> MAHHHHHHMQTYINPPLSEWKNLIQRPVQKAEDLQNIVLTVFEDIKNEKDKALINYTKKFDKAYLTDIRVSSDEITAAIALVSDELIQAIQMAASNIEKFHASQKENKNIIETTEGVNCWREARPIENIGIYIPGGSAPLFSTVLMLGIPAQLAGCKNITLCTPPDESGNINPAILYTANLIGIKNIYKAGGIQAIGAMTFGTETIEKADKIFGPGNQYVTAAKQIAQNFGVAIDMPAGPSEVLVIADTTANPEFVAADLLSQAEHGADSQVILLTTDENILQQTLMQVENQLTQLPRKSIASQALLQSRGIVLDS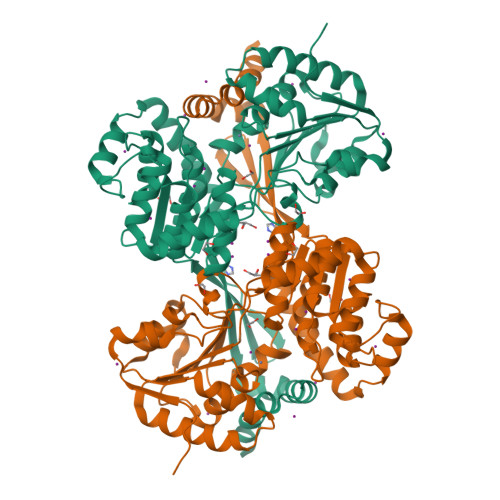IEKCIAFSNLYAPEHLILAIENTENYTDKITSAGSVFLGNFSCESAGDYASGTNHTLPTNGYARNYSGVSLDSFIKKITFQKVTKKGIQNIGPGIEKMAEAEELFAHKHAVSVRLKSLNSQNNTLIKDEKF>[6x]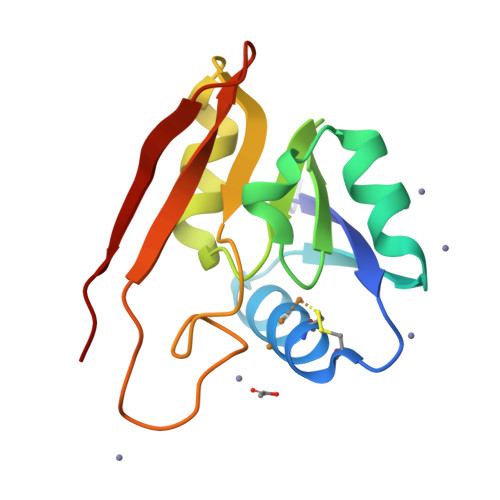EPLAIDVHRDANCGCCKDWIKHLEANGFKVTDHVEADMSAVKSRLGVPYSMGSCHTGVIDGKFVEGHVPAADILKLRERADLVGAAVPGMPVGSPGMEMGDRQDAYQVVGLTRSGQASVLAEYPGR2-cyclohexyl-N-[(3-{[(2,4,6-trimethylphenyl)carbamoyl]amino}naphthalen-2-yl)carbonyl]-D-alanine | C30 H35 N3 O4 | 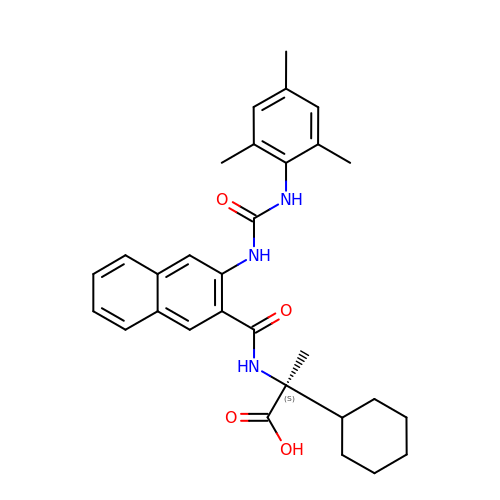ZYHGLTOSKWXGQM-PMERELPUSA-N> ATSDSNMLLNYVPVYVMLPLGVVNVDNVFEDPDGLKEQLLQLRAAGVDGVMVDVWWGIIELKGPKQYDWRAYRSLLQLVQECGLTLQAIMSFHQCGGNVGDIVNIPIPQWVLDIGESNHDIFYTNRSGTRNKEYLTVGVDNEPIFHGRTAIEIYSDYMKSFRENMSDFLESGLIIDIEVGLGPAGELRYPSYPQSQGWEFPGIGEFQCYDKYLKADFKAAVARAGHPEWELPDDAGKYNDVPESTGFFKSNGTYVTEKGKFFLTWYSNKLLNHGDQIL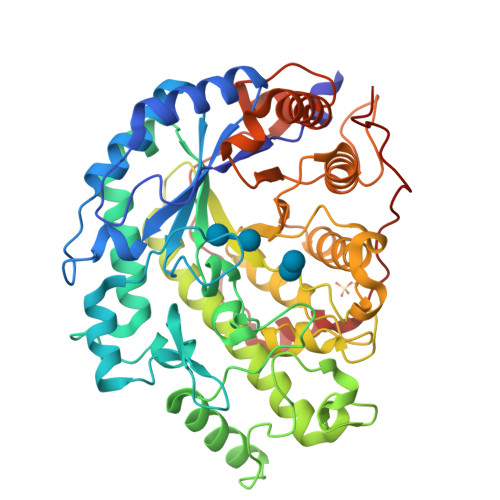DEANKAFLGCKVKLAIKVSGIHWWYKVENHAAELTAGYYNLNDRDGYRPIARMLSRHHAILNFTCLEMRDSEQPSDAKSGPQELVQQVLSGGWREDIRVAGQNALPRYDATAYNQIILNARPQGVNNNGPPKLSMFGVTYLRLSDDLLQKSNFNIFKKFVLKMHADQDYCANPQKYNHAITPLKPSAPKIPIEVLLEATKPTLPFPWLPETDMKVDG Nylon hydrolase (NylC) is one of the three enzymes responsible for the endo-type degradation of the by-products of nylon-6 manufacture (cyclic and linear oligomers of 6-aminohexanoate (Ahx) with a degree of polymerization greater than three) and various aliphatic nylons (e.g., nylon-6 and nylon-66). However, the post-translational autocleavage of the nascent polypeptide between Asn266 and Thr267 generates an active enzyme with an α subunit (27 kDa) and a β subunit (9 kDa). Based on the X-ray-crystallographic structure of NylCA, we reported that four αβ heterodimers (molecules A-D) form a doughnut-shaped quaternary structure. In addition, we proposed that the nucleophilic N-terminal residue Thr267 in the β subunit functions as a catalytic residue for either autocleavage (from precursor to active enzyme) or substrate hydrolysis.

To extensively analyze the effect of amino acid substitution at position 122, we constructed 10 new mutants in which Asp122 of NylCp2 was replaced with other amino acids by site-directed mutagenesis. The values of Tm (melting point of the heat denaturation) and ΔH (change in enthalpy for the global unfolding of proteins) were determined by regression analysis using nonlinear least-squares fitting of the CD melting curve. The Tm values increased in the order of Asp122 (wild-type NylCp2) < Leu < Gln < Asn < Arg < Lys < Val < Gly and ranged from 52.9 °C to 75.1 °C (type 1 mutation in Fig. 2). However, the D2 symmetry was partly altered by mutations at position 122. Plotting the protein stability (Tm value) estimated from the CD analyses against the distance between the two monomer molecules revealed that the protein stability exhibited an inverse correlation with the a2/a1 ratio (index of symmetry). In other words, the ratio changed from 0.979 to 1.197 from the wild-type (Asp122) to the mutant (Arg122, Lys122, Val122, and Gly122) enzyme, although this value should be equal to one for a perfectly symmetric structure. A clearer correlation was found between thermostability and the nearest distance between the side-chain atoms on helix α2 and helix α1. Notably, this distance decreased with an almost linear correlation with increasing thermostability in the wild-type and mutant enzymes.

>[2x]MNTTPVHALTDIDGGIAVDPAPRLAGPPVFGGPGNDAFDLAPVRSTGREMLRFDFPGVSIGAAHYEEGPTGATVIHIPAGARTAVDARGGAVGLSGGYDFNHAICLAGGAGYGLEAGAGVSRALLERLEHRTGFAELQLVSSAVIYDFSARSTAVYPDKALGRAALEFAVPGEFPQGRAGAGMSASAGKVDWDRTEITGQGAAFRRLGDVRILAVVVPNPVGVIVDRAGTVVRGNYDAQTGVRRHPVFDYQEAFAEQVPPVTEAGNTTISAIVTNVRMSPVELNQFAKQVHSSMHRGIQPFHTDMDGDTLFAVTTDEIDLPTTPGSSRGRLSVNATALGAIASEVMWDAVLEAGK> MAAGVAAWLPFARAAAIGWMPVASGPMPAPPRQERKRTQDALIVLNVSGTRFQTWQDTLERYPDTLLGSSERDFFYHPETQQYFFDRDPDIFRHILNFYRTGKLHYPRHECISAYDEELAFFGLIPEIIGDCCYEEYKDRRRENAERLQDDADTDTAGESALPTMTARQRVWRAFENPHTSTMALVFYYVTGFFIAVSVIANVVETVPCGSSPGHIKELPCGERYAVAFFC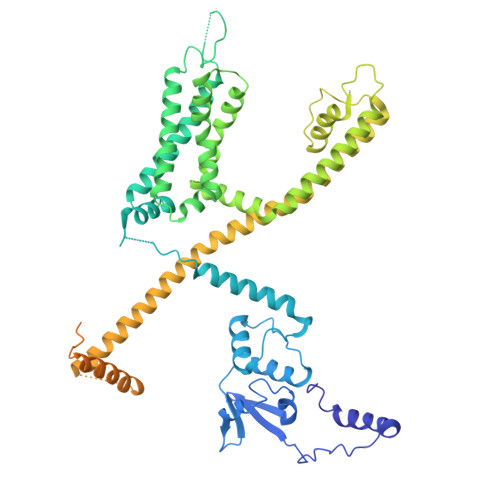LDTACVMIFTVEYLLRLAAAPSRYRFVRSVMSIIDVVAILPYYIGLVMTDNEDVSGAFVTLRVFRVFRIFKFSRHSQGLRILGYTLKSCASELGFLLFSLTMAIIIFATVMFYAEKGSSASKFTSIPAAFWYTIVTMTTLGYGDMVPKTIAGKIFGSICSLSGVLVIALPVPVIVSNFSRIYHQNQRADKRRAQKKARLARIRAAKSGSANAYMQSKRSGLLSNQLQSSEDEPAFVSKSGSSFETQHHHLLHCLEKTTNHEFVDEQVFEESCMEVATVNRPSSHSPSLSSQQGVTSTCCSRRHKKTFRIPNANVSGSHRGSVQELSTIQIRCVERTPLSNSRSSLNAKMEECVKLNCEQPYVTTAIISIPTPPVTTPEGDDRPESPEYSGGNIVRVSAL>[6x]MATLATKKATLVAALKDLQRVTVAFSGGIDSTLVLKMALDVLGRDNVTAVVANSELFTDEEFDKAMSLAEELGANVQGTTLDYLSDDHIKNNTPDSWYYAKKMFYSRLNDIAANNGSAAVLDGMIKNDENDYRPGLKARSEAGARSLLQEADFFKTDVRALAQELGLTNWNKVASCSVSSRFPYGTTLTHDNIAQVMAAEKYLRSLGFPTVRVRFHNDIARIELPEARIGDFLVFNDRVNRQLQSLGFRYVTLDLGGFRSGRMNDTLTKAQLATFAASWSHPQFEK

Nevertheless, the tri-Asp site in LarE represents an unusual metal binding site that selectively and stoichiometrically binds certain multivalent cations. In the apoprotein structure the tri-Asp site is pre-formed to receive a metal ion by a hydrogen bond network consisting of Asp231, Arg228, Gly207, and several water molecules filling the site. Notably, the arginine residues form a positively charged ring around the tri-Asp site, limiting the metal-Asp interactions along the three-fold symmetry axis and likely responsible for only one metal ion being captured by these residues. We observed binding to the tri-Asp site for Ca2+, Mn2+, both Fe2+ and Fe3+, Co2+, Ni2+, Cu2+, Zn2+, and Cd2+, whereas Mg2+, K+, Cr3+, Cu+ and Cs+ did not bind at that location (data not shown).

In all cases, the Asp231 side chains bind the metals with bidentate coordination, with a seventh site always showing extra density that we modelled as a water molecule. Nevertheless, the best interpretation of electron density is always a seven-coordinated metal atom consistent across all observed elements. For small molecule complexes in the Cambridge Structural Database (CSD) the most common and second most frequent coordination numbers for Mn2+, Fe2+/3+, Co2+, Ni2+, Zn2+, and Cd2+ are 6 and 4; while for Ca2+ they are 6 and 7; and for Cu2+ they are 5 and 635. The results show a similar picture for these elements with the most frequent coordination number being 6 for Mn, Fe, Co, and Ni; 7 (closely followed by 6) for Ca; and 4 for Cu, Zn, and Cd (with 6 coordination being less frequently observed). Interestingly, when carboxyl groups are involved in chelating Zn2+ or Cd2+ in protein structures, 7 coordination (as observed in LarE) is actually the most frequently observed coordination. Several metal soaks (Co, Ni, Zn, and Cd) also resulted in binding of these metals to surface exposed residues. These partially disordered sites only appeared after metal soaks, showing a significant electron density peak and in some cases anomalous peaks. In most cases the surface site involved only a single histidine residue. This resulted in higher B-factors of these metals compared to the tri-Asp site. We reason that the tri-Asp site captures low levels of contaminating metal ions, most likely Ni, Co, or Cd, from the Superdex 200 resin used for other protein purifications in the laboratory.>[2x]MGNDDIRQVYYRDKGISHAKAGRYSQAVMLLEQVYDAD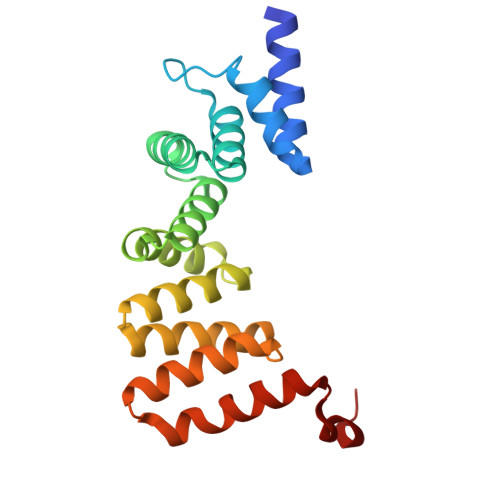AFDVDVALHLGIAYVKTGAVDRGTELLERSLADAPDNVKVATVLGLTYVQVQKYDLAVPLLIKVAEANPINFNVRFRLGVALKNLGRFDEAIDSFKIALGLRPNEGKVHRAIAFSYEQMGRHEEALPHFKKANELDEGASVELALVPR> MSDGNVAWILASTALVMLMVPGVGFFYAGMVRRKNAVNMIALSFISLIITVLLWIFYGYSVSFGNDISGIIGGLNYALLSGVKGEDLLFMMYQMMFAAVTIAILTSAIAERAKVSSFILLSALWLTFVYAPFAHWLWGGGWLAKLGALDFAGGMVVHISSGFAALAVAMTIGKRAGFEEYSIEPHSIPLTLIGAALLWFGWFGFNGGSALAANDVAINAVVVTNTSAAVAGFVWMVIGWIKGKPGSLGIVSGAIAGLAAITPAAGFVDVKGAIVIGLVAGIVCYLAMDFRIKKKIDESLDAWAIHGIGGLWGSVAVGILANPEVNGYAGLLFGNPQLLVSQLIAVASTTAYAFLVTLILAKAVDAAVGLR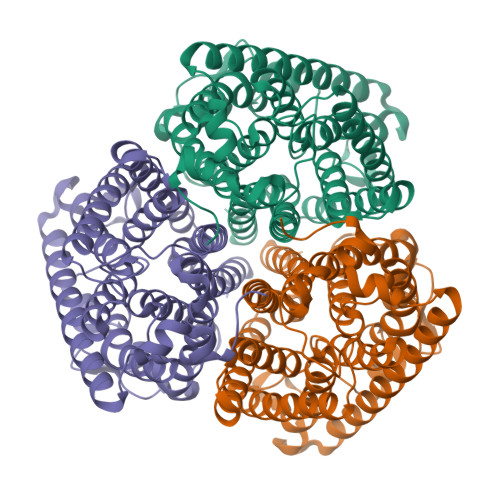VSSQEEYVGLDLSQHEEVAYTLEHHHHHH> QEHHHHHHSSGLVPRGSGQESVTMDGKQYSTIEVNGQTYLIPDNGSKKRVARSLDS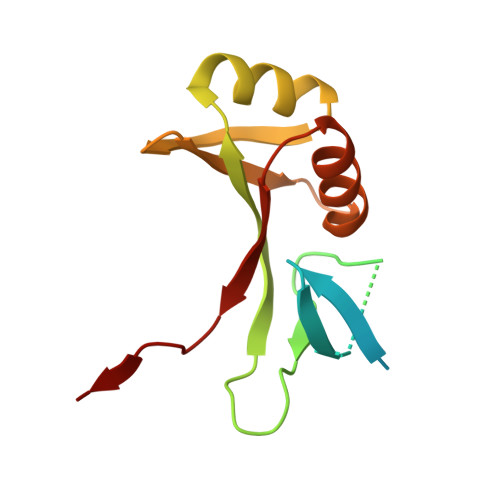KVPQQTLRRGDVLMQGAASPELTVSGTLLVEADDASAKALATRHGLNFKQSSGGIALLEAKPGTDLNAIATKLKSEGVNVQIELSGAEQQPK> GPL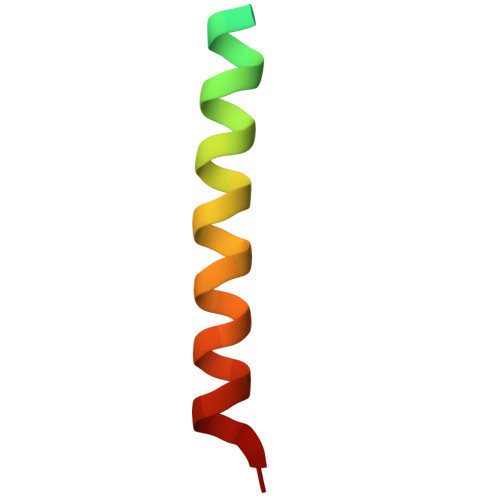GSASARTANPTAKRQFVQSAKEVANSTANLVKTIKAL> MAATAAEAVASGSGEPREEAGALGPAWDESQLRSYSFPTRPIPRLSQSDPRAEELIENEEPVVLTDTNLVYPALKWDLEYLQENIGNGDFSVYSASTHKFLYYDEKKMANFQNFKPRSNREEMKFHEFVEKLQDIQQRGGEERLYLQQTLNDTVGRKIVMDFLGFNWNWINKQQGKRGWGQLTSNLLLIGMEGNVTPAHYDEQQNFFAQIKGYKRCILFPPDQFECLYPYPVHHPCDRQS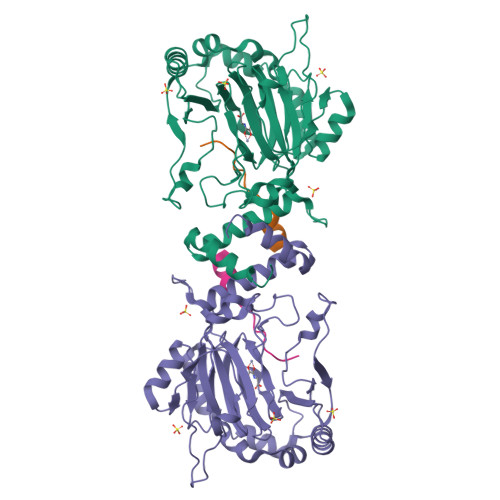QVDFDNPDYERFPNFQNVVGYETVVGPGDVLYIPMYWWHHIESLLNGGITITVNFWYKGAPTPKRIEYPLKAHQKVAIMRNIEKMLGEALGNPQEVGPLLNTMIKGRYN;> HLEVVKLLLEHGADVSAQDK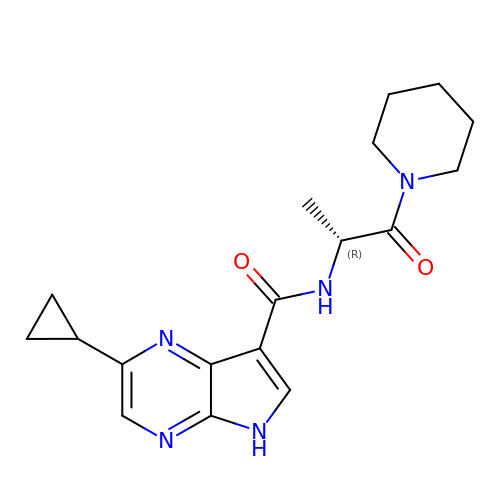2-cyclopropyl-N-[(2R)-1-oxo-1-(piperidin-1-yl)propan-2-yl]-5H-pyrrolo[2,3-b]pyrazine-7-carboxamide | C18 H23 N5 O2 | STEKXUJMQOKLQV-LLVKDONJSA-N> 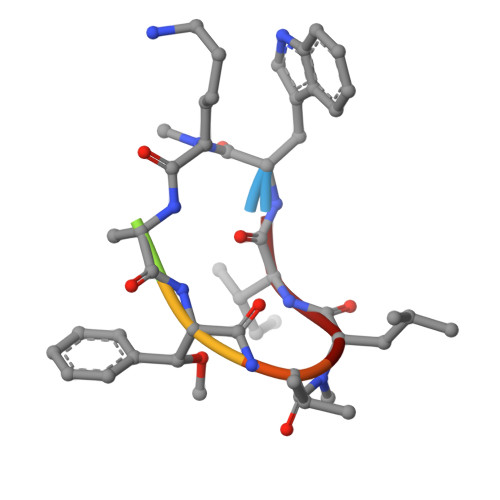WXAFVLI>[2x]MSVRDEFDAWAADGRDKGMEDRHWHTAKHALARMPVEEGDTVVDLGTGSGYALRALRDTKGIGRGFGL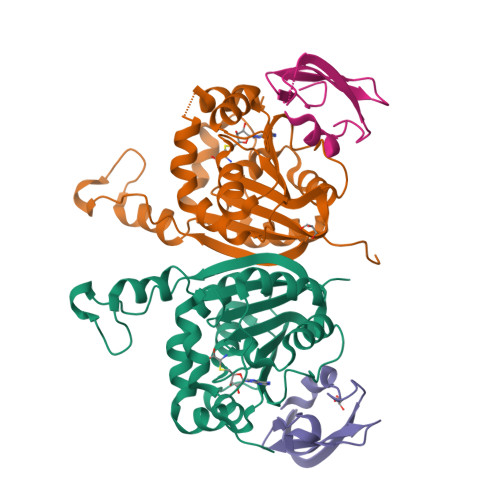DGSPEMVQNARAYTDTDDLSFLVGDFDDLPFDDDSVDHVWSMEAFYYAADPHHTLEEIARILKPGGTFYCAVNYYEENVHSHEWQEHISIDMTRWSHAEYREAFRDAGLHVAEQDSIADLDIDIPAATEFPTDDWETREAMVERYRTFGTLLTVGVAPHHHHH;>MKESLMDILCDPLDKSELELEVDERDGDEIIEGRLIGTVTGEVYPIEDGIPNLLPPDMRDD[2x]>GSGSMKDYDELLKYYELHETIGTGGFAKVKLACHILTGEMVAIKIMDKNTLGSDLPRIKTEIEALKNLRHQHICQLYHVLETANKIFMVLEYCPGGELFDYIISQDRLSEEETRVVFRQIVSAVAYVHSQGYAHRDLKPENLLFDEYHKLKLIDFGLCAKPKGNKDYHLQTCCGSLAYAAPELIQGKSYLGSEADVWSMGILLYVLMCGFLPFDDDNVMALYKKIMRGKYDVPKWLSPSSILLLQQMLQVDPKKRISMKNLLNHPWIMQDYNYPVEWQSKNPFIHLDDDCVTELSVHHRNNRQTMEDLISLWQYDHLTATYLLLLAKKARGKPVRLRLSSFSCG[2x]

Maternal embryonic leucine zipper kinase (MELK) is a serine/threonine kinase in the adenosine monophosphate-activated protein kinase (AMPK)-related kinase family, and was first identified as a maternal gene in mouse eggs and preimplantation embryos. Out of all of these potential roles, MELK is best characterized as a mitotic kinase, as its expression pattern highly correlates with other mitotic genes. At the protein level, MELK is hyperphosphorylated, and reaches its maximal abundance and kinase activity during M phase in both Xenopus embryos and human cancer cell lines. Due to the potential oncogenic role of MELK, several groups have developed MELK inhibitors to validate its potential as a drug target.

Lastly, MRT199665, a pan-AMPK-related kinase inhibitor, showed reasonable potency against MELK (IC50 = 29 nM). To better understand the mode of inhibitor binding, we determined crystal structures of MELK in complex with HTH-01-091 and MRT199665. The MRT199665 structure also revealed a type I binding mode. The pyrimidine and aniline nitrogen atoms from the core form dual hydrogen bonds with the backbone NH and carbonyl group of Cys89 in the hinge. Toward the deep pocket, MRT199665 hydrogen bonds with Lys40, while the dimethyl group abuts the gatekeeper L86, promoting a relatively open conformation of the N-lobe. The hydroxy group of the hydroxydihydroindene group forms a hydrogen bond with Glu93, restricting the plane of the indene orthogonoal to the rest of the molecule. The indene group is in van der Waals contact with Gly18 and Val25, but intervening residues in the P-loop are largely disordered. Specifically, the pyrrolopyrimidine MRT199665 induced MELK degradation most efficiently. We postulate that the induced conformation upon binding of MRT199665 is more poised for the degradation response.In addition to the shared TMD-DH catalytic core of NOX, the functional DUOX protein has an additional large N-terminal extracellular peroxidase homology domain (PHD) and a long intracellular loop 0 containing two EF-hand domains, and it requires an auxiliary DUOXA protein for proper function. The activity of DUOX is regulated by intracellular calcium concentration. hDUOX1 subunits and hDUOXA1 subunits co-assemble into a 2:2 heterotetrameric protein complex with molecular weight ~457 kDa. Here, we present the cryo-EM structures of human DUOX1–DUOXA1 (hDUOX1–hDUOXA1) complex in both high-calcium and low-calcium states, providing insights into the structure and mechanism of calcium activation for DUOX.

We prepared cryo-EM grids using the peptidisc sample, either in the presence of 2.5 mM ethylene glycol tetraacetic acid (EGTA; low calcium) or 0.5 mM free calcium (high calcium). The overall resolution of cryo-EM maps in the low-calcium and high-calcium states reached 2.7 and 2.6 Å, respectively. In the high-calcium state, individual domains of DUOX1 in the cytosolic layer are stabilized by multiple inter-domain interactions. The PHLD interacts with adjacent TMD and DH domains. The EF1–EF2 module in the high-calcium state shapes a crevice that embraces α4 and post α4 loop of the DH domain. The interactions between the EF module and DH are mainly hydrophobic and involve F768, F772, F807, F819, F840, and F847 of the EF module, L1463, M1467, I1470, F1475, V1478, and F1484 of the DH domain. DH docks onto the bottom of TMD via polar interaction between R1270 on M6 and D1367 on β7, and between R1113 on loop B of TMD and N1550 of DH. Moreover, both the FAD cofactor and NADPH substrate bind at the interface between DH and TMD. The measured edge-to-edge distances between NADPH and FAD, between FAD and inner heme, and between inner heme and outer heme are 8.2, 3.9, and 6.7 Å, respectively. The structure of hDUOX1 complex in the high-calcium state reveals multiple inter-domain interactions that orientate DH and TMD for electron transfer, and thus redox reaction.

>[2x]MGFCLALAWTLLVGAWTPLGAQNPISWEVQRFDGWYNNLMEHRWGSKGSRLQRLVPASYADGVYQPLGEPHLPNPRDLSNTISRGPAGLASLRNRTVLGVFFGYHVLSDLVSVETPGCPAEFLNIRIPPGDPMFDPDQRGDVVLPFQRSRWDPETGRSPSNPRDPANQVTGWLDGSAIYGSSHSWSDALRSFSRGQLASGPDPAFPRDSQNPLLMWAAPDPATGQNGPRGLYAFGAERGNREPFLQALGLLWFRYHNLWAQRLARQHPDWEDEELFQHARKRVIATYQNIAVYEWLPSFLQKTLPEYTGYRPFLDPSISSEFVAASEQFLSTMVPPGVYMRNASCHFQGVINRNSSVSRALRVCNSYWSREHPSLQSAEDVDALLLGMASQIAEREDHVLVEDVRDFWPGPLKFSRTDHLASCLQRGRDLGLPSYTKARAALGLSPITRWQDINPALSRSNDTVLEATAALYNQDLSWLELLPGGLLESHRDPGPLFSTIVLEQFVRLRDGDRYWFENTRNGLFSKKEIEEIRNTTLQDVLVAVINIDPSALQPNVFVWHKGDPCPQPRQLSTEGLPACAPSVVRDYFEGSGFGFGVTIGTLCCFPLVSLLSAWIVARLRMRNFKRLQGQDRQSIVSEKLVGGMEALEWQGHKEPCRPVLVYLQPGQIRVVDGRLTVLRTIQLQPPQKVNFVLSSNRGRRTLLLKIPKEYDLVLLFNLEEERQALVENLRGALKESGLSIQEWELREQELMRAAVTREQRRHLLETFFRHLFSQVLDINQADAGTLPLDSSQKVREALTCELSRAEFAESLGLKPQDMFVESMFSLADKDGNGYLSFREFLDILVVFMKGSPEEKSRLMFRMYDFDGNGLISKDEFIRMLRSFIEISNNCLSKAQLAEVVESMFRESGFQDKEELTWEDFHFMLRDHNSELRFTQLCVKGVEVPEVIKDLCRRASYISQDMICPSPRVSARCSRSDIETELTPQRLQCPMDTDPPQEIRRRFGKKVTSFQPLLFTEAHREKFQRSCLHQTVQQFKRFIENYRRHIGCVAVFYAIAGGLFLERAYYYAFAAHHTGITDTTRVGIILSRGTAASISFMFSYILLTMCRNLITFLRETFLNRYVPFDAAVDFHRLIASTAIVLTVLHSVGHVVNVYLFSISPLSVLSCLFPGLFHDDGSEFPQKYYWWFFQTVPGLTGVVLLLILAIMYVFASHHFRRRSFRGFWLTHHLYILLYVLLIIHGSFALIQLPRFHIFFLVPAIIYGGDKLVSLSRKKVEISVVKAELLPSGVTHLRFQRPQGFEYKSGQWVRIACLALGTTEYHPFTLTSAPHEDTLSLHIRAAGPWTTRLREIYSAPTGDRCARYPKLYLDGPFGEGHQEWHKFEVSVLVGGGIGVTPFASILKDLVFKSSVSCQVFCKKIYFIWVTRTQRQFEWLADIIREVEENDHQDLVSVHIYITQLAEKFDLRTTMLYICERHFQKVLNRSLFTGLRSITHFGRPPFEPFFNSLQEVHPQVRKIGVFSCGPPGMTKNVEKACQLINRQDRTHFSHHYENF;>[2x]MATLGHTFPFYAGPKPTFPMDTTLASIIMIFLTALATFIVILPGIRGKTRLFWLLRVVTSLFIGAAILAVNFSSEWSVGQVSTNTSYKAFSSEWISADIGLQVGLGGVNITLTGTPVQQLNETINYNEEFTWRLGENYAEEYAKALEKGLPDPVLYLAEKFTPRSPCGLYRQYRLAGHYTSAMLWVAFLCWLLANVMLSMPVLVYGGYMLLATGIFQLLALLFFSMATSLTSPCPLHLGASVLHTHHGPAFWITLTTGLLCVLLGLAMAVAHRMQPHRLKAFFNQSVDEDPMLEWSPEEGGLLSPRYRSMADSPKSQDIPLSEASSTKAYYRPRRLSLVPADVRGLAPAALSALPGALLAQAWRALLPGLRCPKAGKESRLGPPHSPWRFGPEGCEERWAEHTGDSPRPLRGRGTGRLWRWGSKERRACGVRAMLPRLVSNSGLKRPSCLDLPKCWDYRRDARAFFHLLEPTPCVTSRHTPLI> PPPP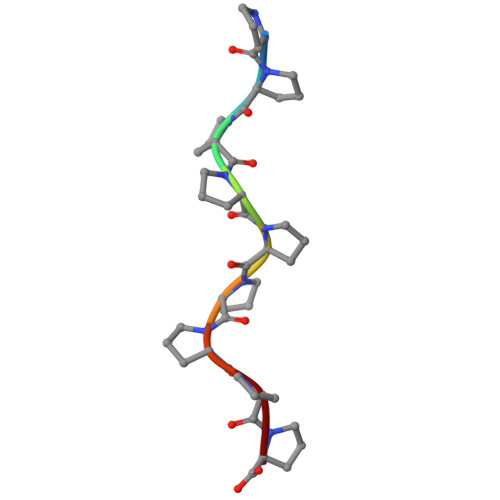PPPPP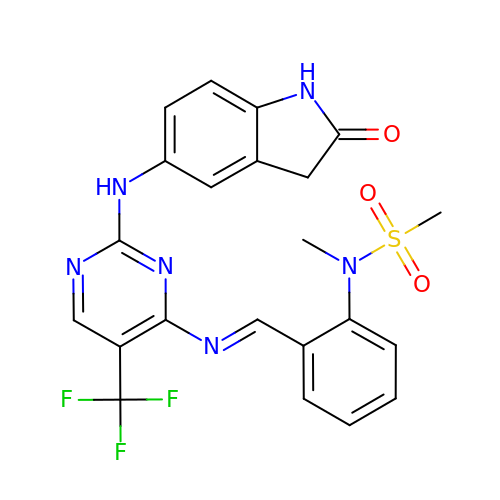N-Methyl-N-(2-{[2-(2-oxo-2,3-dihydro-1H-indol-5-ylamino)-5-trifluoromethyl-pyrimidin-4-ylamino]-methyl}-phenyl)-methanesulfonamide | C22 H19 F3 N6 O3 S | MONLGZGTNBTOCO-KBKYJPHKSA-N We identified C12orf29 (RLIG1) as an atypical ATP-grasp enzyme. Our biochemical and structural characterizations revealed this enzyme to be a 5’ to 3’ RNA ligase, structurally and functionally similar to phage T4 RNA ligase. Although the 5’ to 3’ RNA ligases contain the ATP-grasp fold, their catalytic mechanism is different from canonical members of this superfamily; they transfer an AMP moiety from ATP to the side-chain amino group of an active-site lysine to form a ligase-(lysyl-N)-AMP intermediate. To gain insight into the reaction mechanism of RLIG1, we solved crystal structures of WT (adenylated) and K73M Yasminevirus sp. GU-2018 (28) RLIG1 (YspRLIG1) in the presence of ATP.

In the YspRLIG1K73M structure, ATP was bound in the active site. Both structures were virtually identical; thus, we use the YspRLIG1K73M structure to describe the interactions related to catalysis. YspRLIG1K73M clamps the ATP molecule with two antiparallel β-sheets, a common feature of the ATP-grasp fold and the RNA ligase superfamily. We superimposed the active sites of ADP-bound YspRLIG1WT with ATP-bound YspRLIG1K73M. The pyrophosphate group of the ATP from the YspRLIG1K73M structure is not poised for catalysis because the Lys73 (Motif I) is replaced with a Met and is 6.4 Å from the Pα of the ATP (Nζ-Pα-O3α angle = 85.4°). Arg89 (Motif Ia) coordinates ATP-binding and forms a hydrogen bond with the 3’-OH of the ribose ring. Glu174 (Motif III), His195 (Motif IIIa), and the 2’-OH of the ribose ring form a hydrogen bonding network that precisely orients the nucleotide in the active site. Lys253 (Motif V) is involved in neutralizing the negative charge from the nucleotide. Superposition of the YspRLIG1K73M and T4 Rnl1 active sites suggests that Asp75 (Motif I), Glu174 (Motif III), Glu240 (Motif IV), and Lys253 (Motif V) may be involved in Mg2+ binding. Collectively, our structural analyses of YspRLIG1 reveal a minimal and atypical RNA ligase fold and highlight key active site residues involved in RNA ligation.

>[6x]SMSDMNSESKSNTVSDKMCEVHDKISAILVCAHVKGTETEKAGRSGEKYLATNCLNPGLISAIQAGARVVPTAMTDGTCCRVFNGKIQKRRDIKPGREVPEGWIQTGSDEKSGHLIGFMDLEKGDKWHYDCHVKDPSSPSGLDINKVLCITTNKAGDALVYEEVNIADLNGHTVELMGPKFQSNPHGLKAHCLMRHGTVKLTDFPDLRDYVSVDGAEPLKENALADIRNWFLNSKQGPHLEGVVLHLDNGEMYKLHRHHLDLEWSAKSARPLDQIPL> SEFCSEADATIVIKQWNQIYNAGIGAKSR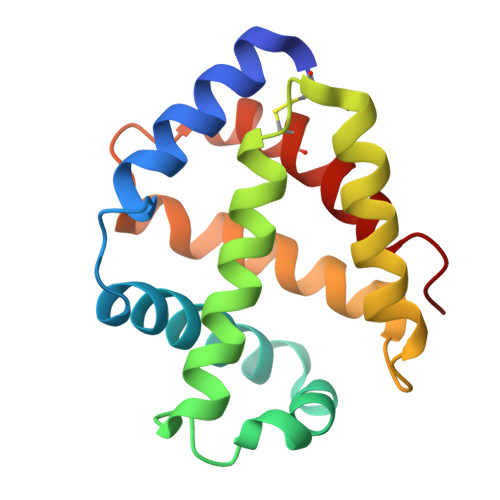WTMGNEIFSSLFKLKPESEVLFNNVNVANMSSGAFHAHTVRVLSGLDMGINYLNDAGTLTSLTAHLAAQHVARTGLKAVYFDAMGKVLMTVLPSLIDNFNPDAWRNCLLPLKNAIAKGLP>[12x]PIVDSGSVAPLSAAEKTKIRSAWAPVYSNYETSGVDILVKFFTSTPAAQEFFPKFKGMTSADQLKKSADVRWHAERIINAVN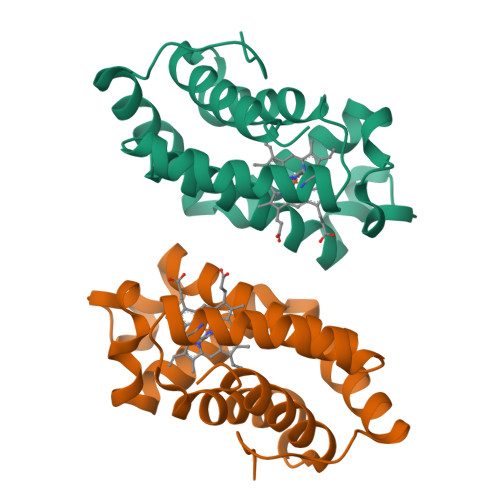DAVASMDDTEKMSMKLRDLSGKHAKSFQVDPQYFKVLAAVIADTVAAGDAGFEKLMSMICILLRSAY>[6x]MATLATKKATLVAALKDLQRVTVAFSGGIDSTLVLKMALDVLGRDNVTAVVANSELFTDEEFDKAMSLAEELGANVQGTTLDYLSDDHIKNNTPDSWYYAKKMFYSRLNDIAANNGSAAVLDGMIKNDENDYRPGLKARSEAGARSLLQEADFFKTDVRALAQELGLTNWNKVASASVSSRFPYGTTLTHDNIAQVMAAEKYLRSLGFPTVRVRFHNDIARIELPEARIGDFLVFNDR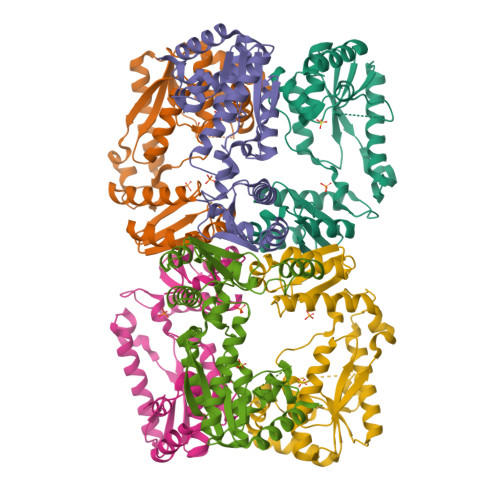VNRQLQSLGFRYVTLDLGGFRSGRMNDTLTKAQLATFAASWSHPQFEK(2S)-1-(nonanoyloxy)-3-(phosphonooxy)propan-2-yl 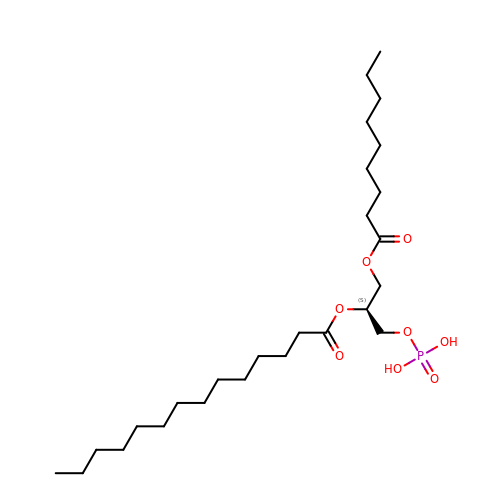tetradecanoate | C26 H51 O8 P | GDXQVZUHVZYLSC-DEOSSOPVSA-N>MHHHHHHEGELKTIMGQAKVSKLQEKMKLDPRSKITFNDFKGIAKEVGIEEKEINSVSNALAQSGSIIYLPNSLNENLKTSVFTKP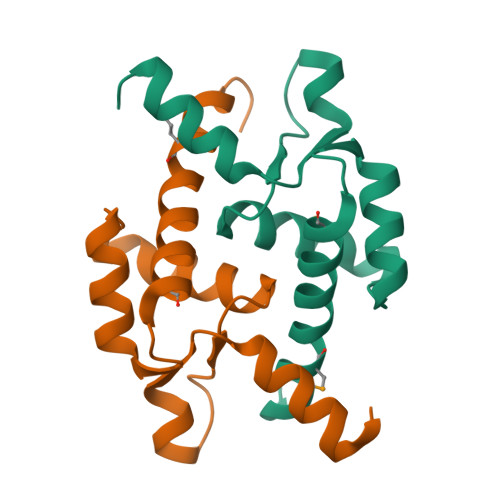AHIYQSLEHILDIENKGVG[4x]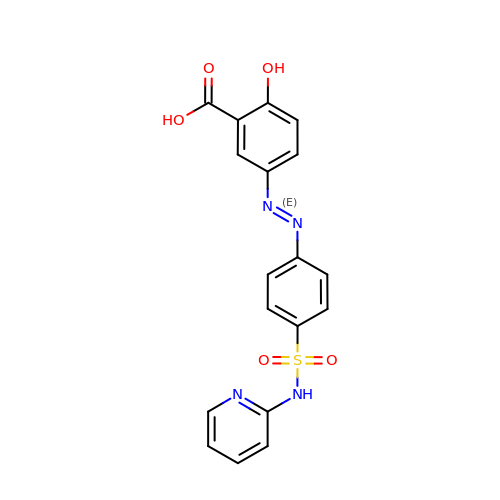2-HYDROXY-(5-([4-(2-PYRIDINYLAMINO)SULFONYL]PHENYL)AZO)BENZOIC ACID | C18 H14 N4 O5 S | NCEXYHBECQHGNR-QZQOTICOSA-N> MERYENLFAQLNDRREGAFVPFVTLGDPGIEQSLKIIDTLIDAGADALELGVPFSDPLADGPTIQNANLRAFAAGVTPAQCFEMLALIREKHPTIPIGLLMYANLVFNNGIDAFYARCEQVGVDSVLVADVPVEESAPFRQAALRHNIAPIFICPPNADDDLLRQVASYGRGYTYLLSRSGVVGAENRGALPLHHLIEKLKEYHAAPALQGFGISSPEQVSAAVRAGAAGAISGSAIVKII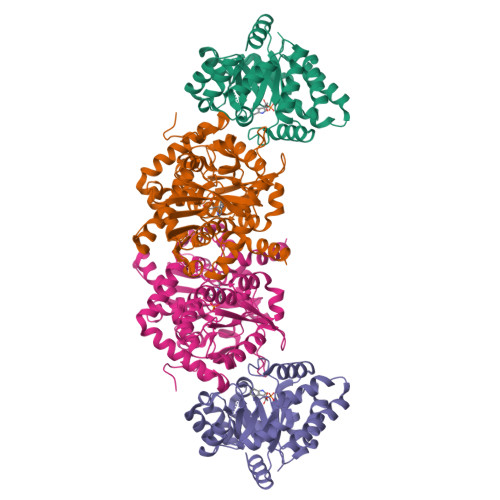EKNLASPKQMLAELRSFVSAMKAASRA;> TTLLNPYFGEFGGMYVPQILMPALNQLEEAFVSAQKDPEFQAQFADLLKNYAGRPTALTKCQNITAGTRTTLYLKREDLLHGGAHKTNQVLGQALLAKRMGKSEIIAETGAGQHGVASALASALLGLKCRIYMGAKDVERQSPNVFRMRLMGAEVIPVHSGSATLKDACNEALRDWSGSYETAHYMLGTAAGPHPYPTIVREFQRMIGEETKAQILDKEGRLPDAVIACVGGGSNAIGMFADFINDTSVGLIGVEPGGHGIETGEHGAPLKHGRVGIYFGMKAPMMQTADGQIEESYSISAGLDFPSVGPQHAYLNSIGRADYVSITDDEALEAFKTLCRHEGIIPALESSHALAHALKMMREQPEKEQLLVVNLSGRGDKDIFTVHDILKARGEI>[8x]MRGSHHHHHHGSAQDLTNMPSLAPVLKNAMPAIVNVAVQGYLPNNMASGNADDDDGENSKQPSR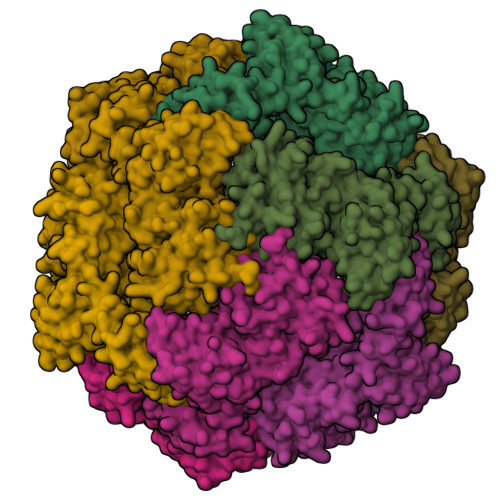IPEKGRKFESIGSGVIIDPKNGIIITNDHVIRNANLITVTLQDGRRLKARLIGGDSETDLAVLKIDAKNLKSLVIGDSDKLEVGDYVVAIGNPFGLNSFGNSQSATFGIVSALKRSDLNIEGVENFIQTDAAINPGNAGGALVNAKGELIGINTAIISPYGGNVGIGFAIPINMAKDVAQQIIKFGSIHRGLMGIFVQHLTPELAQSMGYAEDFQGALVSQVNQNSPAQLAGLKSGDVIVQINDTKITQATQVKTTISLLRAGSTAKIKILRDNKPLTLDVEVTDIKKHEQKLQSNNPFLYGLALRNFEQESPPHGNVVGVQVVGASETSAGWRAGLRPGDIIISANKTPVKDIKSLQAVAHEKGKQLLVQVLRGAGALYLLII> QKQYWVCNSSDASISYTYCDKMQYPISINVNPCIELKGSKGLLHIFYIPRR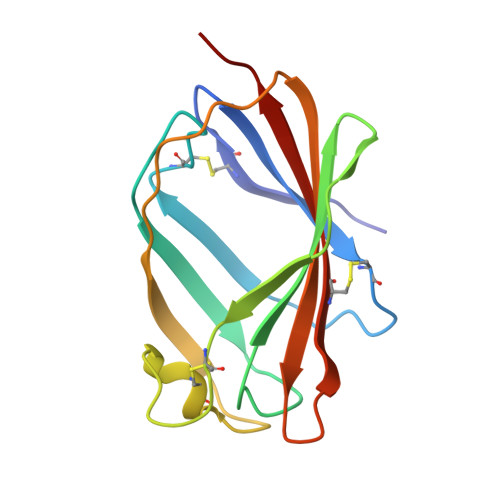DLKQLYFNLYITVNTMNLPKRKEVICRGSDDDYSFCRALKGETVNTTISFSFKGIKFSKGKYKCVVEAISGSPEEMLFCLEFVILHQPNSN> HKCDITLQEIIKDLNSLTEQKTLCTELTVTDIFAASKNTTEKETFCRAATVLRQFYSHHEKDTRCLGATAQQFHRH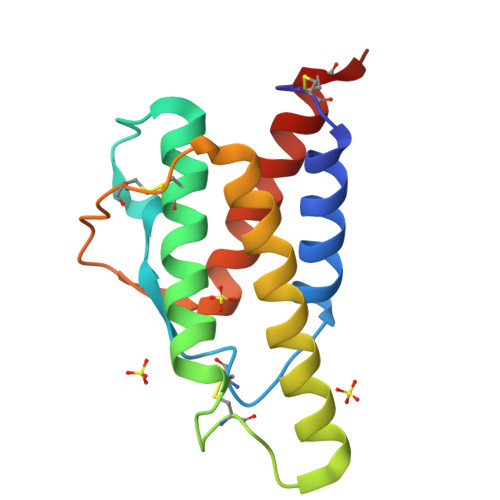KQLIRFLKALDRNLWGLAGLNSCPVKEANQSTLENFLERLKTIMREKYSKCSS> QSEPELKLESVVIVSRAGVRAPTKATQLMQDVTPDAWPTWPVKLGWLTPRGGELIAYLGHYQRQRLVADGLLAKKGCPQSGQVAIIADVDERTRKTGEAFAAGLAPDCAITVHTQTDTSSPDPLFNPLKTGVCQLDNANVTDAILSRAGGSIADFTGHRQTAFRELERVLNFPQSNLCLKREKQDESCSLTQALPSELKVSADNVSLTGAVSLASMLTEIFLLQQAQGMPEPGWGRITDSHQWNTLLSLHNAQFYLLQRTPEVARSRATPLLDLIKTALTPHPPQKQAYGVTLPTSVLFIAGHDTNLANLGGALELNWTLPGQPDNTPPGGELVFERWRRLSDNSQWIQVSLVFQTLQQMRDKTPLSLNTPPGEVKLTLAGCEE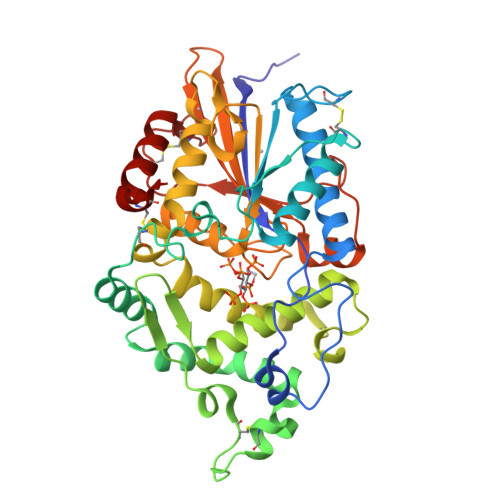RNAQGMCSLAGFTQIVNEARIPACSL>MIQIYHADAFEIIKDFYQQNLKVDAIITDPPYNISVKNNFPTLKSAKRQGIDFGEWDKNFKLLEWIARYAPLVNPNGCMVIFCSYRFISYIADFLEENGFVVKDFIQWVKNNPMPRNIHRRYVQDTEFALWAVKKKAKWVFNKPKNEKYLRPLILKSPVVSGLEKTKHPTQKSLALMEKIISIHTNPNDIVLDPFMGSGTTGLACKNLERNFIGIESEKEYFQTAKKRL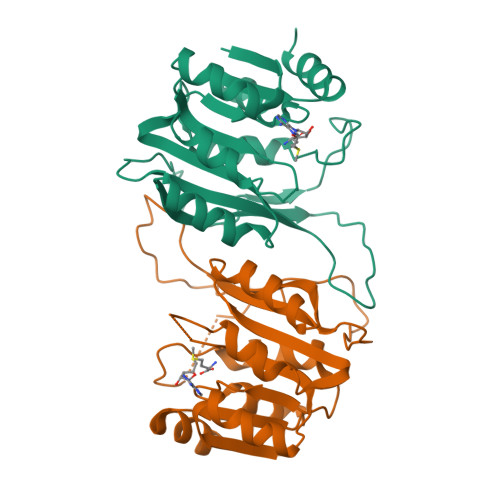NLF[8x]>MDSHCRVRPAGPAVPADCDPPRITHAALAARLGDARLLTLYDQATWSEGPAWWEAQRTLVWSDLVGRRVLGWRED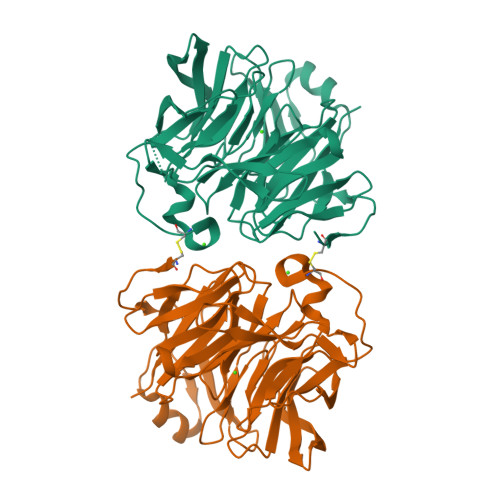GTVDVLLDATAFTNGNAVDAQQRLVHCEHGRRAITRSDADGQAHLLVGRYAGKRLNSPNDLIVARDGAIWFTDPPFGLRKPSQGCPADPELAHHSVYRLPPDGSPLQRMADLDHPNGLAFSPDEQTLYVSQTPEQGHGSVEITAFAWRDGALHDRRHFASVPDGLPDGFCVDRGGWLWSSSGTGVCVFDSDGQLLGHIPTPGTASNCTFDQAQQRLFITGGPCLWMLPLP[2x]>[4x]ASMTGGQQMGRDEAGITGTWYNQLGSTFIVTAGADGALTGTYESAVGNAESRYVLTGRYDSAPATDGSGTALGWTVAWKNNY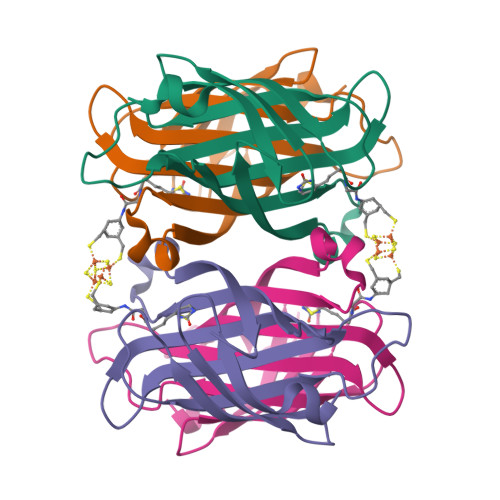RNAHSATTWSGQYVGGAEARINTQWLLTAGTTEANAWASTLVGHDTFTKVKPSAASIDAAKKAGVNNGNPLDAVQQ> MILHALTQYYQRKAESAQKGICLVTGKAAPIARLHNAVKGVNAKPAPFASVNLSAFESYGKEQGFAFPIGEQAMFEYTTALNTLLAGENRFRIGDVTTVCWGAKRTPLEESLASMINGGGKDKPDEHIDAVKTLYKSLYNGQYQKPDGKEKFYLLGLSP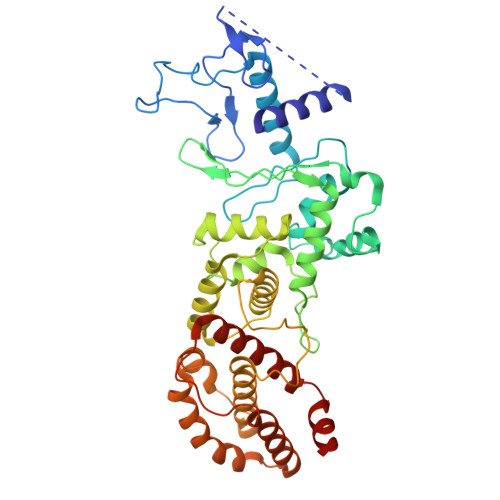NSARIVVRFWHETTVAALSESIAAWYDDLQMVRGENSPYPEYMPLPRLLGNLVLDGKMENLPSDLIAQITDAALNNRVLPVSLLQAALRRNKAEQKITYGRASLLKAYINRAIRAGRLKNMKELTMGLDRNRQDIGYVLGRLFAVLEKIQAEANPGLNATIADRYFGSASSTPIAVFGTLMRLLPHHLNKLEFEGRAVQLQWEIRQILEHCQRFPNHLNLEQQGLFAIGYYHETQFLFTKDALKNLFNEA> MAATAAEAVASGSGEPREEAGALGPAWDESQLRSYSFPTRPIPRLSQSDPRAEELIENEEPVVLTDTNLVYPALKWDLEYLQENIGNGDFSVYSASTHKFLYYDEKKMANFQNFKPRSNREEMKFHEFVEKLQDIQQRGGEERLYLQQTLNDTVGRKIVMDFLGFNWNWINKQQGKRGWGQLTSNLLLIGMEGNVTPAHYDEQQNFFAQIKGYKRCILFPPDQFECLYPYPVHHPCDRQSQVDFDNPDYERFPNFQNVVGYETVVGPGDVLYIPMYWWHHIESLLNGGITITVNFWYKGAPTPKRIEYPLKAHQKVAIMRNIEKMLGEA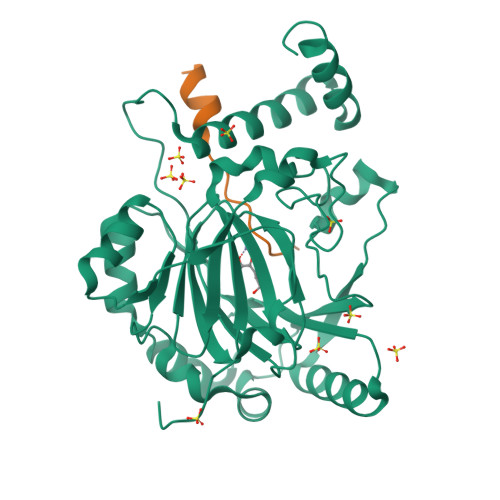LGNPQEVGPLLNTMIKGRYN;> HLEVVKLLLEAGADVNAQDK(2~{R})-2-[[(2~{S})-2-[[(4~{R})-5-azanyl-4-[[(2~{S})-2-azanylpropanoyl]amino]-5-oxidanylidene-pentanoyl]amino]-6-[2-[2-[2-[2-(2-azanylethanoylamino)ethanoylamino]ethanoylamino]ethanoylamino]ethanoylamino]hexanoyl]amino]propanoic 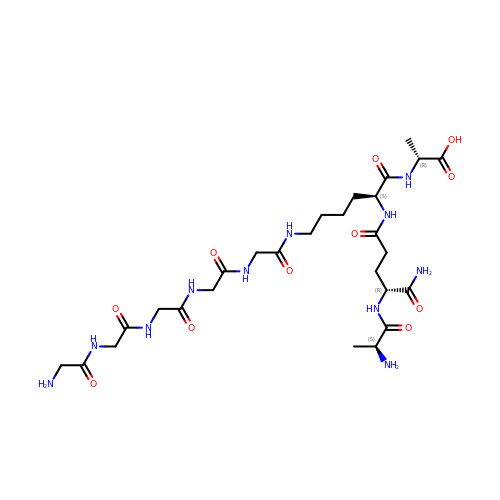acid | C27 H47 N11 O11 | HUYIRRKHPBSVEV-HZMVEIRTSA-N> SMEMYETLGKVGEGSYGTVMKCKHKNTGQIVAIKIFYERPEQSVNKIAMREIKFLKQFHHENLVNLIEVFRQKKKIHLVFEFIDHTVLDELQHYCHGLESKRLRKYLFQILRAIDYLHSNNIIHRDIKPENILVSQSGITKLCDFGFARTLAAPGDIYDDEVATRWYRAPELVLKDTSYGKPVDIWALGCMIIEMATGNPYLPSSSDLDLLHKIVLKVGNLSPHLQNIFSKSPIFAGVVLPQVQHPKNARKKYPKLNGLLADIVHACLQIDPADRISSSDLLHHEYFTRDGFIEKFMPELKAKLLQEAKVNSLIKPKESSKENEL

Here, we present the crystal structures of human CDKL1, CDKL2, CDKL3, and CDKL5, revealing their evolutionary divergence from CDK and mitogen-activated protein kinases (MAPKs), including an unusual αJ helix important for CDKL2 and CDKL3 activity. CDKL family proteins contain a conserved N-terminal kinase domain and variable C termini. The kinase domains of CDKL1, CDKL2, CDKL3, and CDKL5 were crystallized using a phosphomimetic Asp-X-Glu (DXE) substitution and in the presence of identified inhibitors. The CDKL structures all contain broad spectrum ATP-competitive inhibitors that bind to the kinase hinge region via 3 hydrogen bonds.

By contrast, the CDKL1, CDKL3, and CDKL5 structures displayed characteristics of active kinases. Inhibitor ASC67 was designed as an affinity reagent (Statsuk et al., 2008) and was among the top screening hits for all CDKLs tested. Its nitrile H bonded with the catalytic lysines of CDKL3 and CDKL5. Catalytic site interactions may help support the active conformation of these kinases. Instead, CDKL2 and CDKL3 showed an unusual amphipathic helix, αJ, while the constructs for CDKL1 and CDKL5 were truncated and lacked this region. Notably, deleting the αJ region reduced the activities of CDKL2 and CDKL3, whereas CDKL1 and CDKL5 were largely unchanged. These results are consistent with the observed structures, and they further show the importance of the unprecedented αJ helix for CDKL2 and CDKL3 function.>[5x]MADRI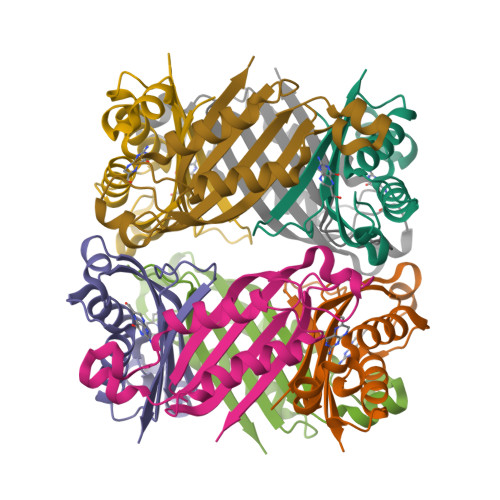ELRGLTVHGRHGVYDHERVAGQRFVIDVTVWIDLAEAANSDDLADTYDYVRLASRAAEIVAGPPRKLIETVGAEIADHVMDDQRVHAVEVAVHKPQAPIPQTFDDVAVVIRRSR;>[2x]MADRIELRGLTVHGRHGVYAHERVAGQRFVIDVTVWIDLAEAANSDDLADTYDYVRLASRAAEIVAGPPRKLIETVGAEIADHVMDDQRVHAVEVAVHKPQAPIPQTFDDVAVVIRRSR;> MADRIELRGLTVHGRHGVAAHERVAGQRFVIDVTVWIDLAEAANSDDLADTYDYVRLASRAAEIVAGPPRKLIETVGAEIADHVMDDQRVHAVEVAVHKPQAPIPQTFDDVAVVIRRSR>MSTVGTGKLTRAQRRAAARKNKRNTRVVQPVIVEPIASGQGKAIKAWTGYSVSKWTASCAAAEAKVTSAITISLPNELSSERNKQLKVGRVLLWLGLLPSVSGTVKSCVTETQTTAAASFQVALAVADNSKDVVAAMYPEAFKGITLEQLAADLTIYLYSSAALTEGDVIVHLEVEHVRPTFDDSFTPVY[6x]

The spherical cowpea chlorotic mottle virus (CCMV, diameter d = 28 nm) is one of the most studied viruses. Its 180 capsid protein (CP) copies are arranged into 20 hexamers and 12 pentamers, resulting in a quasi-icosahedral T = 3 symmetry. The complexation process is driven by protein–protein interactions and by electrostatic interactions between the negatively charged phosphate backbone of the DNA origami and the positively charged amino acid (aa) residues (+9) in the 26-residue arginine-rich N-terminal region of the protein (190 aa, ~20 kDa). Due to the CPs’ innate protein assembly pathways, reassembly results in the formation of hexagonal sheets, empty spheres and tubes.

After characterizing the starting materials (dimensions are given as average (avg) ± s.d. throughout), 6HB (davg = 6.1 ± 0.6 nm) and intact CCMV (davg = 26.8 ± 1.0 nm) with negative-stain transmission electron microscopy (TEM), the complexation of isolated CPs and 6HB was performed at physiological conditions (pH 7.3, 150 mM NaCl) using the CPs in excess. Negative-stain TEM images and small-angle X-ray scattering (SAXS) for samples complexed at ε = 2k (6HB-2k) reveal 6HB complexes with increased diameter due to a highly ordered protein shell (bottom), which develops from nucleation sites along the origami structure (ε < 2k). Two-dimensional (2D) classification of particles picked along the filaments and 3D refinement of ab initio 3D models, obtained from the recorded images only, results in helical structures with 4.3 Å resolution (left) for the first protein layer and 8 Å resolution for the second protein layer. The protein tubes are assembled of hexamers (top right), similar to tubes formed by in vitro assembled human immunodeficiency virus (HIV). Whereas the first layer is characterized by a 1-start helix with a turn of 63.8° and a rise of 15.4 Å, the second layer has a 3-start helical symmetry with a turn of 38.8° and a 29.6 Å rise. The density in the lumen of the protein tubes corresponds to the encapsulated DNA origami. N-termini facing the origami create a positive electrostatic potential surface for the inner surface of the protein tube (bottom right). For the outer tube surface, in contrast, the negative electrostatic potential is predominant (top right), hence allowing the formation of protein multilayer complexes. We were not able to detect a specific physical contact point between the protein layers, or between DNA and protein, suggesting that unspecific electrostatic and protein–protein interactions were the driving force for the assembly. The cryo-EM densities of CPs encapsulating 6HB clearly show large holes between the hexameric units, resembling the swollen state, which is expected according to the solution conditions used.>[2x]MASREEIFSKVKSIISEKLGVDESQVTEEAKLIDDLGADSLDLVDLVMDFESEFGVKVDDADLEKISTVGDIVSYIEKKLG

Acyl carrier proteins (ACPs) are small (~9 kDa) acidic proteins that are essential for numerous biochemical pathways, including the biosynthesis of fatty acids, polyketides, lipopolysaccharides, lipoteichoic acids, rhizobial nodulation signaling factors, and pro-hemolysin toxins. As essential components in type II FAS systems, ACPs shuttle acyl intermediates in their hydrophobic pocket to facilitate interactions with various enzyme partners. ACPs consist of four helical bundles connected by three loop regions, forming hydrophobic cavities to accommodate the growing acyl chains. In this respect, Thermotoga maritima ACP (Tm-ACP) is a valuable target since T. maritima resides in extremely hot hydrothermal vents and is the only bacterium known to grow at temperatures up to 90 °C. Its thermophilic cell membrane is highly enriched in saturated fatty acids with long chain lengths, which help maintain their liquid crystalline states at high temperatures.

To function as a carrier for acyl groups, an apo Tm-ACP should be converted to the holo form, where the phosphopantetheine linker is covalently connected to the side chain of S40 in the conserved DSL motif. Both tertiary structures of the holo and apo forms of Tm-ACP were determined by NMR spectroscopy and X-ray crystallography, respectively (see associated statistics in Table 2). Tm-ACP consists of four α-helices (helix I (4–19), helix II (40–54), helix III (60–65), helix IV (69–80)) connected by a long α1α2 loop and two shorter loops. Compared to the structure of holo Ec-ACP, the helix III of Tm-ACP was found to be protruded outward in both the apo and holo forms. Hyperthermophilic Tm-ACP has nonconserved Glu and Lys residues (D59 and K79), which participate in an ionic cluster between helices III and IV, forcing the outward protrusion of helix III. The Tm-ACP structure has extensive electrostatic interactions in four different regions. The interior of Tm-ACP is filled with numerous hydrophobic side chains, in which three Phe residues and I15 mediate the tight hydrophobic packing. The specific Tm of Tm-ACP was measured as 101.4 °C by DSC, which is the highest melting temperature for any ACP reported to date. For hyperthermophilic Tm-ACP, the distances between the Cα atoms of the corresponding residues, L43, L63, and S67, were increased to 8.6 Å, 7.5 Å, and 9.1 Å, respectively, forming a much larger entrance. This would facilitate the entrance of long acyl chains into the hydrophobic pocket of Tm-ACP.> MISKYRYLHCARKLVKQSVQAFGGGHHHHEYDWRDDPKVNKDIEEDIRDRGWHPETYDFPYTKKHDDWVFDVTMPSQNYQTDLTVNIHPENKKMHVMKQVMRQ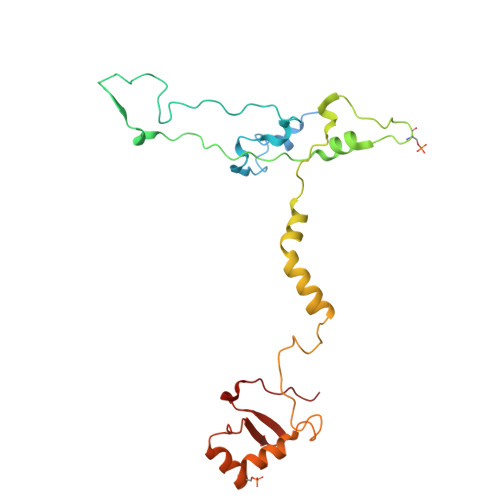SYWDAEHDMAHEYDYESEDLDFQCESFKSQHFRKKGPISQYLILGLLPILYFGTEFFYNHYPDEDYWRVAHPPPLDYPDTDDTDDTETFKDYKSFTGRRMVDTGIVDPLWYDIREGKKVYYDWAGVNQPMEDI>[3x]VIGGTNASPGEFPWQLSQQRQSGSWSHSCGASLLSST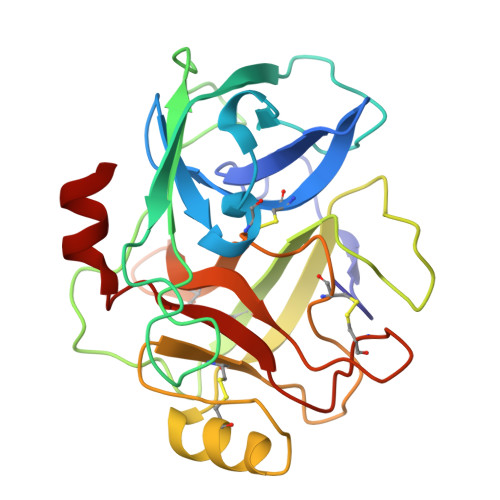SALSASHCVDGVLPNNIRVIAGLWQQSDTSGTQTANVDSYTMHENYGAGTASYSNDIAILHLATSISLGGNIQAAVLPANNNNDYAGTTCVISGWGRTDGTNNLPDILQKSSIPVITTAQCTAAMVGVGGANIWDNHICVQDPAGNTGACNGDSGGPLNCPDGGTRVVGVTSWVVSSGLGACLPDYPSVYTRVSAYLGWIGDNS> SNWDTKFLKKGYTFDDVLLIPAESHVLPNEVDLKTKLADNLTLNIPIITAAMDTVTGSKMAIAIARAGGLGVIHKNMSITEQAEEVRKVKRSENGVIIDPFFLTPEHKVSEAEELMQRYRISGVPIVETLANRKLVGIITNRDMRFISDYNAPISEHMTSEHLVTAAVGTDLETAERILHEHRIEKLPLVDNSGRLSGLITIKDIEKVIEFPHAAKDEFGRLLVAAAVGVTSDTFERAEALFEAGADAIVIDTAHGHSAGVLRKIAEIRAHFPNRTLIAGNIATAEGARALYDAGVDVVKVGIGPGSICTTRVVAGVGVPQVTAIYDAAAVAREYGKTIIADGGIKYSGDIVKALAAGGNAVMLGSMFAGTDEAPGETEIYQGRKYKTYRGMGSIAAMKKGSSDRYFQGSVNEANKLVPEGIEGRVAYKGAASDIVFQMLGGIRSGMGYVG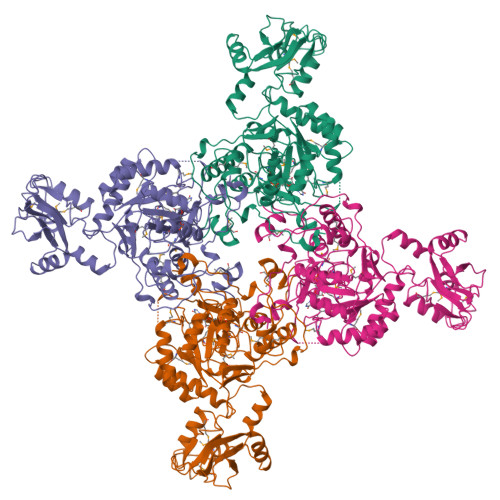AGDIQELHENAQFVEMSGAGLIESHPHDVQITNEAPNYSV>[4x]DPTMSVIKPDMKIKLRMEGAVNGHPFAIEGVGLGKPFEGKQSMDLKVKEGGPLPFAYDILTMAFCYGNRVFAKYPENIVDYFKQSFPEGYSWERSMIYEDGGICIATNDITLDGDC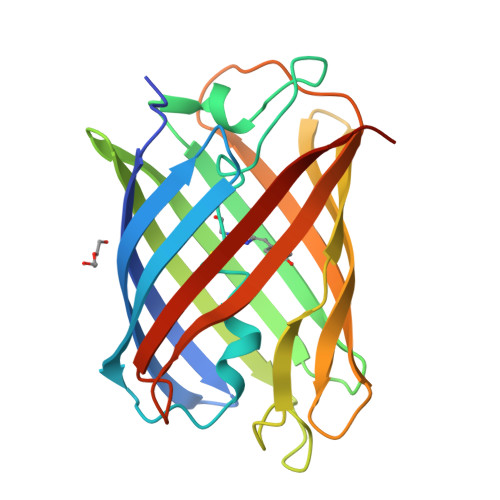YIYEIRFDGVNFPANGPVMQKRTVKWEPSTEKLYVRDGVLKSDGNYALSLEGGGHYRCDSKTTYKAKKVVQLPDYHDVVHHIEIKSHDRDYSNVNLHEHAEAHSGLPRQAKX>GARGSNTIGARLNRVEDKVTQLDQRLALI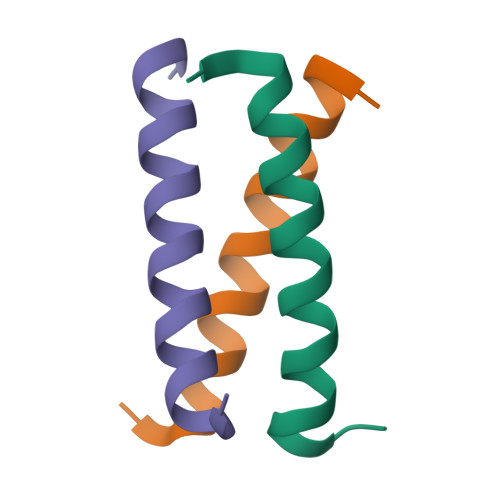TD[3x]Rucaparib 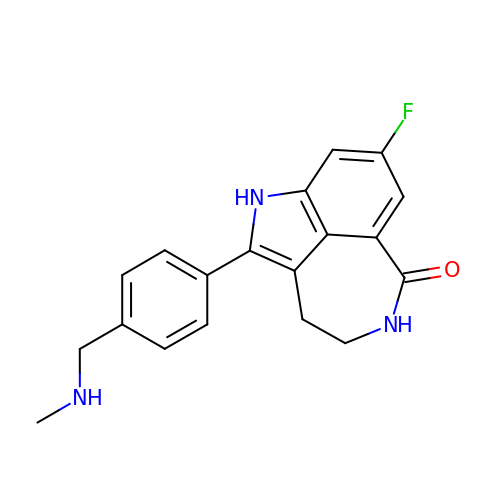| C19 H18 F N3 O | HMABYWSNWIZPAG-UHFFFAOYSA-N> 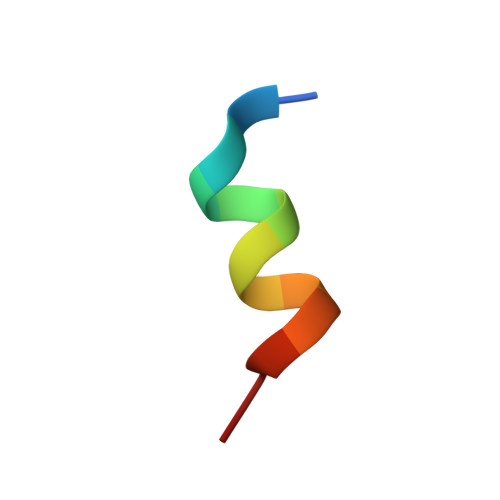VERLQIFQHLHPI> MFAKLHGKKQRPISSINSQTPRTSNTTHANSISLSSGNLIVGSNRNLRQKKEQFGSQQRASGRKLISNKENDDNVNNGGDNNYDNGERVHRHHIPGLKIKAYQAELGYHESRFSENLVMLNLVEFPDIKPGDLVELKTYHKNPSASNGDKKIYFIAKDFDGETKRRAKTSNVSILSGQLQTLLDLPSRSRIWIKLKPNKFDLQADVVEFNIKDCLLNRGDMWVLSSKLVDTCVFMDQRLAFLDSIRGTIKGIYRNGKKIVSGYIGEQTRIIFRSESARLIFLIQITDEMWNFEETGEQLFQKMVNSFFPKIFKKWKDVDTHHTITIAFAISMDLSDTSFKDLTPGESLKNSQDYFRIVVDQVSIIHWVDIMETLREEFMEIRKDLLNKQTDKGYSVANGRFSPVIKSNFLELVNFATTILTDPFKQLDLRHTTTHVMIISPGSGLFDVDYSLLRLTGKKLLSLEMTMDLICLSKAPLHIVPLFRYRDFENKLHHCVPLWLSVFFWNDHDKKSNSEWTPRCKIYDLQMMGITENELIREVDVEYLQLNKKVKSLSEFMNDYDK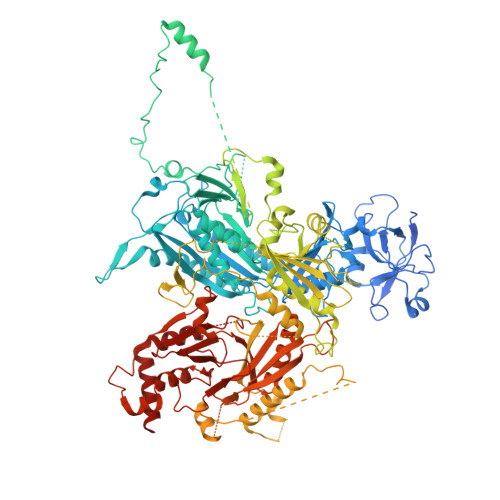NAFEVKILCAGSNTKQSKKLNSKFDTVFENDVVVKARKIPATATTTHGNTKFIWRGPKVALPAIKDIQKPNVIPDLSIKTIEASFYDDCNTTNDKISTPTTSNNDNLEMNDSLVSVRSADNQNTSLALDSLKGLSKRNSLKDFTQRVITKFISNIDTSKNKKIKSTLLRDDVDNSPLGSNTPLPSSESKISGLKLQQKGLADENVISKRGNLIIKKNLSIFGLPSNEIMSGSPSSYLGSSHTRTSSKLSNMSDKAAFITEGQKSKHDDSNTYSLTQQLKHRISETWVDIKSPSIPVSSEFANELLPIRWKDVWPKYVARKYSKWRSFTTPAELPITISDFPSKDDFDRNFIFRNHSVTLNTDQEQYNQTYKDLLRDMIYMRLLTGFQICVGRQVEKIELSRESGESETVVNKYLDFNQNDAFKLYLMIDSEIHRITCSSSGIIDVERYLRKDEANLFDQVPSYIPLVKTRYESSFRDAMIDPLHVKRESLNWNQIDQVLAGYGDNLIDRKWHGFRAKYVVLPTDIPPNTYSMVINGKSETLNPEEIRVEGLRRLIGSITRSRLRTEKEKKGRKTKREEIQPEVMFYTGPLYNFINEQQTSLESSAINFKDSIFVNDNNLLNRNVELSKLAYQIQRGEDRITLVNRKWHWKKHEKCFVGSEMVNWLIRNFSDIDTREDAIKYGQKVMKEGLFVHVLNKHNFLDGHYFYQFSPEYVMDTNKLEKTNSHRSTLSDPKQMLRKASTGSSNDPSAMTPFSSVVPAISASNASVADAKEPSRPILMLSNSLVIDVDPAGKSSKQESCTVHYDRVHNPDHCFHIRLEWLTTTPKLIDDLVGNWSRLCERYGLKMIEIPWEELCTIPSVNPFHSFVEIKLAINPWEDPEFKDRELFAKSKFYYHVYLLKASGFLLDNRASKFLQNQDIEFDIMYSWGKPQFKYVQYIHHTGAYVAELRENGCLFLAPNNIYISRVNPGNIIGKIHSASSSSLDAQKVILNFKSTCLDYQKLRSIFLDAKEMWITGKIVED>[2x]MVDNSRTRPRVGHIQFLNCLPLYWGLARTGTLLDFELTKDTPEKLSEQLVRGDLDIGPVTLVEFLKNADDLVAFPDIAVGCDGPVMACVIVSQVPLDRLDGARVALGSTSRTSVRLAQLLLSERFGVQPDYYTCPPDLSLMMQEADAAVLIGDAALRANMIDGPRYGLDVHDLGALWKEWTGLPFVFAVWAARRDYAEREPVITRKVHEAFLASR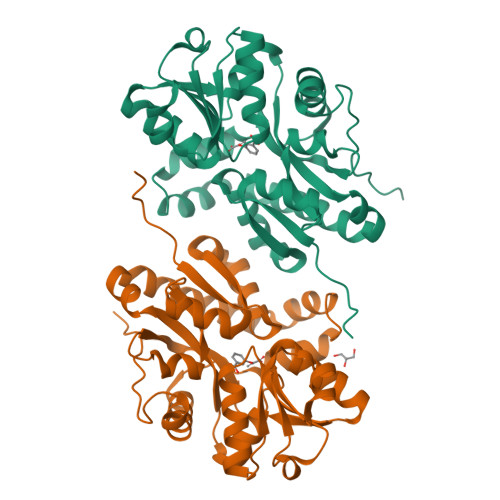NLSLEEVEKVAEQAARWEAFDEDTLAKYFTTLDFRFGAPQLEAVTEFARRVGPTTGFPADVKVELLKPLEHHHHHH>MARQPYRFPQARIPERGSGVFRLTVRNAMAHRDSEMKEECLREDLKFYFMSPCEKYRARRQIPWKLGLQILKIVMVTTQLVRFGLSNQLVVAFKEDNTVAFKHLFLKGYSGTDEDDYSCSVYTQEDAYESIFFAINQYHQLKDITLGTLGYGENEDNRIGLKVCKQHYKKGT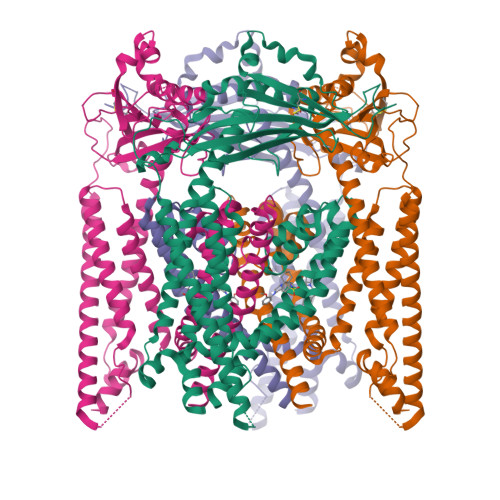MFPSNETLNIDNDVELDCVQLDLQDLSKKPPDWKNSSFFRLEFYRLLQVEISFHLKGIDLQTIHSRELPDCYVFQNTIIFDNKAHSGKIKIYFDSDAKIEECKDLNIFGSTQKNAQYVLVFDAFVIVICLASLILCTRSIVLALRLRKRFLNFFLEKYKRPVCDTDQWEFINGWYVLVIISDLMTIIGSILKMEIKAKNLTNYDLCSIFLGTSTLLVWVGVIRYLGYFQAYNVLILTMQASLPKVLRFCACAGMIYLGYTFCGWIVLGPYHDKFENLNTVAECLFSLVNGDDMFATFAQIQQKSILVWLFSRLYLYSFISLFIYMILSLFIALITDSYDTIKKFQQNGFPETDLQEFLKECSSKEEYQKESSAFLSCICCRRRKRSDDHLIPIS[4x]> MKTMRKQIYKKAYWLLLPFLPLALANTFLVKEDSKNVTAYTPFATPITDSKSDLVSLAQLDSSYQIADQTIHNTNLFVLFKSRDVKVKYESSGSNNISFDSTSQGEKPSYVVEFTNSTNIGIKWTMVKKYQLDVPNVSSDMNQVLKNLILEQPLTKYTLNSSLAKEKGKTQREVHLGSGQANQWTSQRNQHDLNNNPSPNASTGFKLTTGNAYRKLSESWPIYEPIDGTKQGKGKDSSGWSSTEENEAKNDAPSVSGGGSSSGTFNKYLNTKQALESIGILFDDQTPRNVITQLYYASTSKLAVTNNHIVVMGNSFLPSMWYWVVERSAQENASNKPTWFANTNLDWGEDKQKQFVENQLGYKETTSTNSHNFHSKSFTQPAYLISGIDSVNDQIIFSGFKAGSVGYDSSSSSSSSSSSSTKDQALAWSTTTSLDSKTGYKDLVTNDTGLNGPINGSFSIQDTFSFVVPYSGNHTNNGTTGPIKTAYPVKKDQKS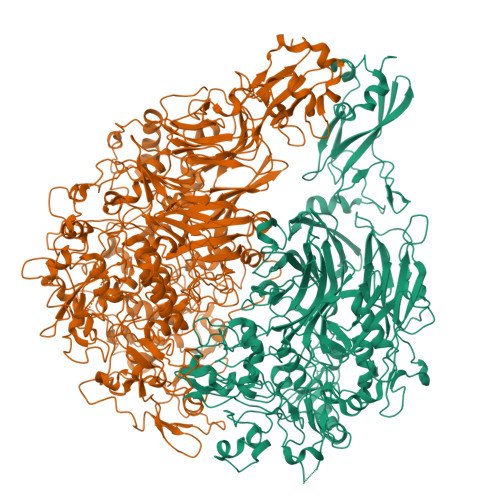TVKINSLINATPLNSYGDEGIGVFDALGLNYNFKSNQERLPSRTDQIFVYGIVSPNELRSAKSSADSTGSDTKVNWSNTQSRYLPVPYNYSEGIIDADGFKRPENRGASVTTFSGLKSIAPDGFANSIANFSVGLKAGIDPNPVMSGKKANYGAVVLTRGGVVRLNFNPGNDSLLSTTDNNIAPISFSFTPFTAAESAVDLTTFKEVTYNQESGLWSYIFDSSLKPSHDGKQTPVTDNMGFSVITVSRTGIELNQDQATTTLDVAPSALAVQSGIQSTTQTLTGVLPLSEEFSAVIAKDSDQNKIDIYKNNNGLFEIDTQLSNSVATNNGGLAPSYTENRVDAWGKVEFADNSVLQARNLVDKTVDEIINTPEILNSFFRFTPAFEDQKATLVATKQSDTSLSVSPRIQFLDGNFYDLNSTIAGVPLNIGFPSRVFAGFAALPAWVIPVSVGSSVGILFILLVLGLGIGIPMYRVRKLQDASFVNVFKKVDTLTTAVGSVYKKIITQTGVVKKAPSALKAANPSVKKPAAFLKPPVQPPSKPEGEQKAVEVKSEETKSHHHHHH;> MHQPKKRLAKKSWAFLTAALTLGVITGVGGYFLFNQNKQRSSVSNFAYQPKQLSVKHQQAVDETLTPWTWNNNNFSSLKITGENPGSFGLVRSQNDNLNISSVTKNSSDDNLKYLNAVEKYLDGQQNFAIRRYDNNGRALYDINLAKMENPSTVQRGLNGEPIFDPFKGFGLTGNAPTDWNEIKGKVPVEVVQSPHSPNLYFVLLVPKVALEYHNLNNQVVKESLEVKATQSSFNPTQRLQKDSPVKDSSKQGEKLSETTASSMSSGMATSTRAKALKVEVERGSQSDSLLKNDFAKKPLKHKNSSGEVKLEAEKEFTEAWKPLLTTDQIAREKGMGATVVSFYDAPYSENHTAFGLVDHIDPKKMVENYPPSWKTPKWNHHGIWDYNARNLLLQTTGFFNPRRHPEWFDEGQAKADNTSPGFKVGDTDHKKDGFKKNSSSPIALPFEAYFANIGNMVAIGNSVFIFGGNGHATKMFTTNPLSIGVFRIKYTDNFSKSSVTGWPYAVLFGGLINPQTNGLKDLPLGTNRWFEYVPRMAVSGVKWVGNQLVLAGTLTMGDTATVPRLKYDQLEKHLNLVAQGQGLLREDLQIFTPYGWANRPDIPVGAWLQDEMGSKFGPHYFLNNPDIQDNVNNDTVEALISSYKNTDKLKHVYPYRYSGLYAWQLFNWSNKLTNTPLSANFVNENSYAPNSLFAAILNEDLLTGLSDKIFYGKENEFAENEADRFNQLLSLNPNPNTNWARYLNVVQRFTTGPNLDSSTFDQFLDFLPWIGNGKPFSNSPSPSTSASSSTPLPTFSNINVGVKSMITQHLNKENTRWVFIPNFSPDIWTGAGYRVQSANQKNGIPFEQVKPSNNSTPFDPNSDDNKVTPSGGSSKPTTYPALPNSISPTSDWINALTFTNKNNPQRNQLLLRSLLGTIPVLINKSGDSNDQFNKDSEQKWDKTETNEGNLPGFGEVNGLYNAALLHTYGFFGTNTNSTDPKIGFKADSSSSSSSTLVGSGLNWTSQDVGNLVVINDTSFGFQLGGWFITFTDFIRPRTGYLGITLSSLQDQTIIWADQPWTSFKGSYLDSDGTPKSLWDPTALKSLPNSSTTYDTNPTLSPSFQLYQPNKVKAYQTTNTYNKLIEPVDATSAATNMTSLLKLLTTKNIKAKLGKGTASSQGNNNGGGVSQTINTITTTGNISEGLKEETSIQAETLKKFFDSKQNNKSEIGIGDSTFTKMDGKLTGVVSTPLVNLINGQGATSDSDTEKISFKPGNQIDFNRLFTLPVTELFDPNTMFVYDQYVPLLVNLPSGFDQASIRLKVISYSVENQTLGVRLEFKDPQTQQFIPVLNASSTGPQTVFQPFNQWADYVLPLIVTVPIVVIILSVTLGLTIGIPMHRNKKALQAGFDLSNKKVDVLTKAVGSVFKEIINRTGISNAPKKLKQATPTKPTPKTPPKPPVKQ> MKTTTPLVHVASVEKGRSYEDFQKVYNAIALKLREDDEYDNYIGYGPVLVRLAWHI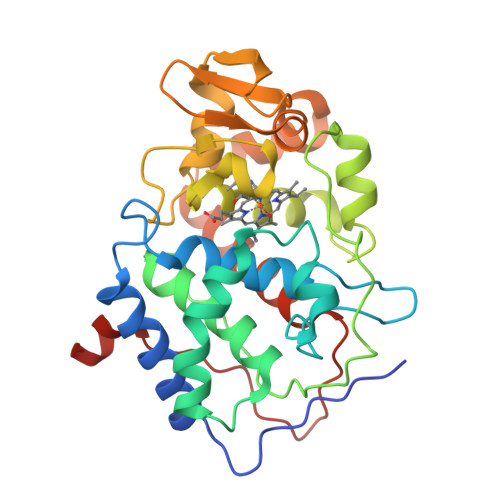SGTWDKHDNTGGSYGGTYRFKKEFNDPSNAGLQNGFKFLEPIHKEFPWISSGDLFSLGGVTAVQEMQGPKIPWRCGRVDTPEDTTPDNGRLPDADKDAGYVRTFFQRLNMNDREVVALMGAHALGKTHLKNSGYEGPWGAANNVFTNEFYLNLLNEDWKLEKNDANNEQWDSKSGYMMLPTEYSLIQDPKYLSIVKEYANDQDKFFKDFSKAFEKLLENGITFPKDAPSPFIFKTLEEQGL>MGSSHHHHHHSSENLYFQGHMLANNNKRSKLSTVPSSRPIRVGFVGLTSGKSWVAKTHFLAIQQLSSQFQIVALYNPTLKSSLQTIEQLQLKHATGFDSLESFAQYKDIDMIVVSVKVPEHYEVVKNILEHSSQNLNLRYLYVEWALAASVQQAEELYSISQQRANLQTIICLQGRKSPYIVRAKELISEGC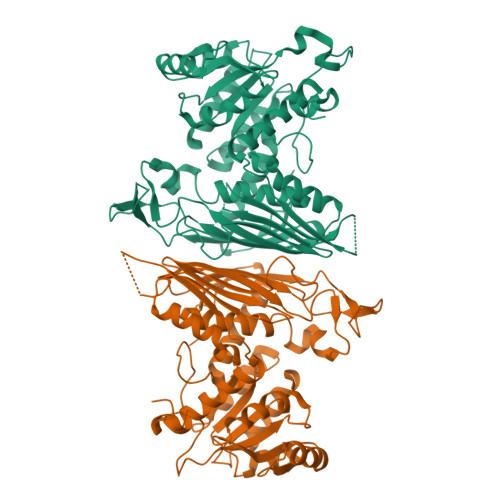IGDINSIEISGNGGWYGYERPMRSPEYLYDIESGVNLISNSFGHTIDVLQYITGSYFQKINAMISNNIPTQFLLDENGKRTKETISKTCPDHLLFQGILENGKVPVSCSFKGGTPVKKLTKNLVIDIHGTKGDLKIEGDAGFVEISNLVLYFYGIKNGNGSSNGTDNNGAAAIKDKEKVTKSPSPSTGTSEEEQTMEVFHLRNYNSVVGNILRIYESIADYHFLGKPESKSSRGPDDLFASTKFDKQGFRFEGFPTFKDAIILHRLIDAVFRSDKEEKTLDVSKIMI[2x]> GSLRVTMNEFEYLKLLGKGTFGKVILVKEKATGRYYAMKI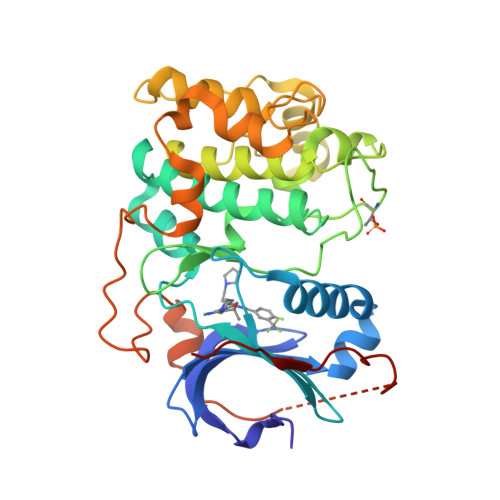LKKEVIVAKDEVAHTLTESRVLQNSRHPFLTALKYSFQTHDRLCFVMEYANGGELFFHLSRERVFSEDRARFYGAEIVSALDYLHSEKNVVYRDLKLENLMLDKDGHIKITDFGLCKEGIKDGATMKTFCGTPEYLAPEVLEDNDYGRAVDWWGLGVVMYEMMCGRLPFYNQDHEKLFELILMEEIRFPRTLGPEAKSLLSGLLKKDPKQRLGGGPSDAKEIMQHRFFAGIVWQHVYEKKLSPPFKPQVTSEVDTRYFDEEFTAQMITITPPDQDDSMECVDSERREEQEMFRDFDYIADWEG1-[3-(4-BROMO-PHENOXY)-PROPOXY]-6,6-DIMETHYL-1.6-DIHYDRO-[1,3,5]TRIAZINE-2,4-DIAMINE 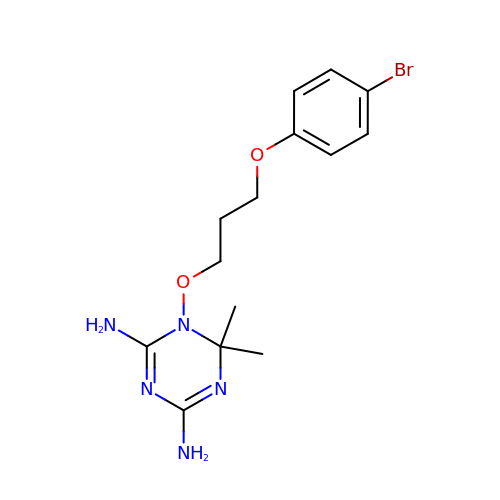| C14 H20 Br N5 O2 | MPXYCOHVHSXSDC-UHFFFAOYSA-N>MQTEHVILLNAQGVPTGTLEKYAAHTADTRLHLAFSSWLFNAKGQLLVTRRALSKKAWPGVWTNSVCGHPQLGESNEDAVIRRCRYELGVEITPPESIYPDFRYRATDPSGIVENEVCPVFAARTTSALQINDDEVMDYQWCDLADVLHGIDATPWAFSPWMVMQATNREARKRLSAFTQLK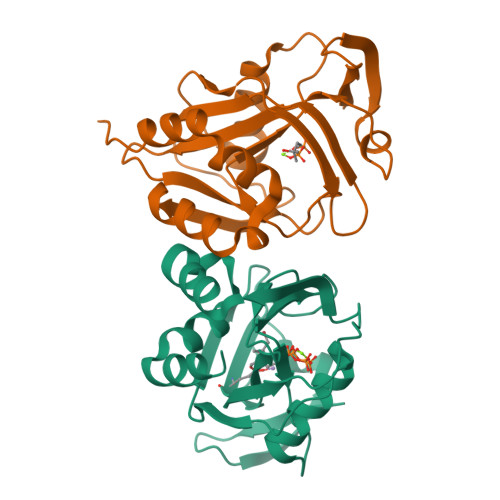LHHHHHH[2x]>[6x]MTSTRLAFAWRELFSVFCYLLYTSDILAERHNNHPVMPICGGISAARIPTADE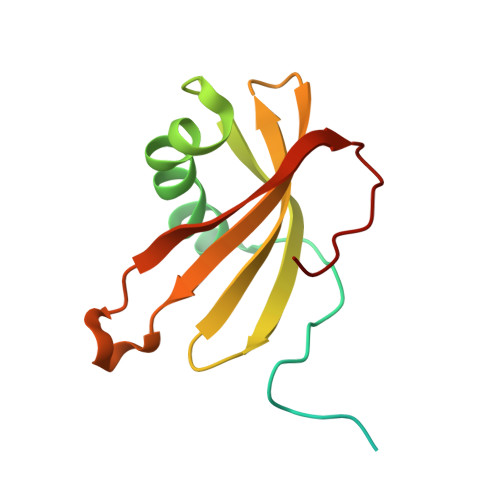KKKLEPVLLQSLYAHLGSKPTSAEVVLVATQVVAGTNYFAKVKVNNDHYIHTRVYEQLPCYGGALELHSVQMNKTDTDPLDYF> MLEQPYLDLAKKVLDEGHFKPDRTHTGTY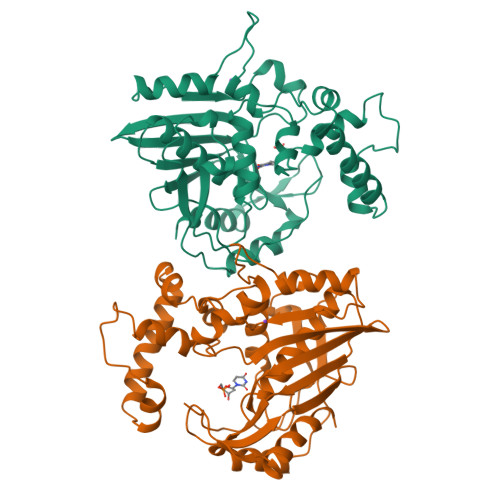SIFGHQMRFDLSKGFPLLTTKKVPFGLIKSELLWFLHGDTNIRFLLQHRNHIWDEWAFEKWVKSDEYHGPDMTDFGHRSQKDPEFAAVYHEEMAKFDDRVLHDDAFAAKYGDLGLVYGSQWRAWHTSKGDTIDQLGDVIEQIKTHPYSTTLIVSAWNPEDVPTMALPPCHTLYQFYVNDGKLSLQLYQRSADIFLGVPFNIASYALLTHLVAHECGLEVGEFIHTFGDAHLYVNHLDQIKEQLSRTPRPAPTLQLNPDKHDIFDFDMKDIKLLNYDPYPAIKAPVAV Here, we addressed the problem of accurate structural validation with cryo-EM-based methodologies for determining the structures of up to megadalton-scale DNA objects in solution, together with molecular-dynamics-based methods for building pseudoatomic models in a semiautomated fashion. The library of objects includes four brick-like multilayer DNA origami objects with increasing internal floppiness, a barrel-like 126-helix bundle, two variants of a multidomain object called Twisttower, a design variant v2 of a previously reported object called the Pointer, a small 16-helix bundle, four variants of a hinged-beam-like object, two variants of a dumbbell-like object, and five variants of a six-helix tube featuring asymmetric markers at either end as reporters for twist and one ten-helix tube. We constructed pseudoatomic models for six different objects. The fitting was validated using Fourier shell correlation against the cryo-EM half-maps and the models show good cross-correlation with the cryo-EM maps.

The Pointer v2 also exhibited other types of structural fluctuations akin to domain motions. These fluctuations are design-specific and depend on the global shape as well as the topology of the nanostructures. As these motions are driven by the thermal fluctuation of the individual helices, they are also dependent on temperature and salt- and buffer conditions, as well as the overall folding quality of the nanostructure ensemble. The heterogeneity may be coarsely classified as relative domain motions similar to those seen in proteins and as helical lattice breathing, which does not exist in proteins.

> ACAAACGGCGGATTGACCGTAATGGTAACCGTAGAGGCGACCACCACC;> TTTTTCGGATTCTCGACCGTATCGGCTTTTT;> TTGACCCCCAGAGCCACGCCACCCTCAGAACCTTTGCTTTTT;> ACTCATCTAAAGTACAGACTCCTCAAGAGAAG;> ACTAAAACATCCGCGATACGTTGGACGGAGATTTGTATCACGCGAAAC;> AAGAATACTAAAGACTGAACTGACGACCTTCAAAATGCAA;> ACGAAGGCACGGGTAAAAATGTGAGGATATTCAGGTCTTT;> TTTTTCTCAGATGCCACTAGGTTGAGGCCATCTTTTCATAAT;> TTTTTATACCAAGTCGTTTTTTTTTTCCTGATAAATT;> TGTAGATGGGCGCATCGGATAGGTCCTGCTCCATGTTACT;> AATGCTACTACTATTAGTAGAATTGATGCCACCTTTTCAGCTCGCGCCCCAAATGAAAATATAGCTAAACAGGTTATTGACCATTTGCGAAATGTATCTAATGGTCAAACTAAATCTACTCGTTCGCAGAATTGGGAATCAACTGTTACATGGAATGAAACTTCCAGACACCGTACTTTAGTTGCATATTTAAAACATGTTGAGCTACAGCACCAGATTCAGCAATTAAGCTCTAAGCCATCCGCAAAAATGACCTCTTATCAAAAGGAGCAATTAAAGGTACTCTCTAATCCTGACCTGTTGGAGTTTGCTTCCGGTCTGGTTCGCTTTGAAGCTCGAATTAAAACGCGATATTTGAAGTCTTTCGGGCTTCCTCTTAATCTTTTTGATGCAATCCGCTTTGCTTCTGACTATAATAGTCAGGGTAAAGACCTGATTTTTGATTTATGGTCATTCTCGTTTTCTGAACTGTTTAAAGCATTTGAGGGGGATTCAATGAATATTTATGACGATTCCGCAGTATTGGACGCTATCCAGTCTAAACATTTTACTATTACCCCCTCTGGCAAAACTTCTTTTGCAAAAGCCTCTCGCTATTTTGGTTTTTATCGTCGTCTGGTAAACGAGGGTTATGATAGTGTTGCTCTTACTATGCCTCGTAATTCCTTTTGGCGTTATGTATCTGCATTAGTTGAATGTGGTATTCCTAAATCTCAACTGATGAATCTTTCTACCTGTAATAATGTTGTTCCGTTAGTTCGTTTTATTAACGTAGATTTTTCTTCCCAACGTCCTGACTGGTATAATGAGCCAGTTCTTAAAATCGCATAAGGTAATTCACAATGATTAAAGTTGAAATTAAACCATCTCAAGCCCAATTTACTACTCGTTCTGGTGTTCTCGTCAGGGCAAGCCTTATTCACTGAATGAGCAGCTTTGTTACGTTGATTTGGGTAATGAATATCCGGTTCTTGTCAAGATTACTCTTGATGAAGGTCAGCCAGCCTATGCGCCTGGTCTGTACACCGTTCATCTGTCCTCTTTCAAAGTTGGTCAGTTCGGTTCCCTTATGATTGACCGTCTGCGCCTCGTTCCGGCTAAGTAACATGGAGCAGGTCGCGGATTTCGACACAATTTATCAGGCGATGATACAAATCTCCGTTGTACTTTGTTTCGCGCTTGGTATAATCGCTGGGGGTCAAAGATGAGTGTTTTAGTGTATTCTTTCGCCTCTTTCGTTTTAGGTTGGTGCCTTCGTAGTGGCATTACGTATTTTACCCGTTTAATGGAAACTTCCTCATGAAAAAGTCTTTAGTCCTCAAAGCCTCTGTAGCCGTTGCTACCCTCGTTCCGATGCTGTCTTTCGCTGCTGAGGGTGACGATCCCGCAAAAGCGGCCTTTAACTCCCTGCAAGCCTCAGCGACCGAATATATCGGTTATGCGTGGGCGATGGTTGTTGTCATTGTCGGCGCAACTATCGGTATCAAGCTGTTTAAGAAATTCACCTCGAAAGCAAGCTGATAAACCGATACAATTAAAGGCTCCTTTTGGAGCCTTTTTTTTTGGAGATTTTCAACGTGAAAAAATTATTATTCGCAATTCCTTTAGTTGTTCCTTTCTATTCTCACTCCGCTGAAACTGTTGAAAGTTGTTTAGCAAAACCCCATACAGAAAATTCATTTACTAACGTCTGGAAAGACGACAAAACTTTAGATCGTTACGCTAACTATGAGGGTTGTCTGTGGAATGCTACAGGCGTTGTAGTTTGTACTGGTGACGAAACTCAGTGTTACGGTACATGGGTTCCTATTGGGCTTGCTATCCCTGAAAATGAGGGTGGTGGCTCTGAGGGTGGCGGTTCTGAGGGTGGCGGTTCTGAGGGTGGCGGTACTAAACCTCCTGAGTACGGTGATACACCTATTCCGGGCTATACTTATATCAACCCTCTCGACGGCACTTATCCGCCTGGTACTGAGCAAAACCCCGCTAATCCTAATCCTTCTCTTGAGGAGTCTCAGCCTCTTAATACTTTCATGTTTCAGAATAATAGGTTCCGAAATAGGCAGGGGGCATTAACTGTTTATACGGGCACTGTTACTCAAGGCACTGACCCCGTTAAAACTTATTACCAGTACACTCCTGTATCATCAAAAGCCATGTATGACGCTTACTGGAACGGTAAATTCAGAGACTGCGCTTTCCATTCTGGCTTTAATGAAGATCCATTCGTTTGTGAATATCAAGGCCAATCGTCTGACCTGCCTCAACCTCCTGTCAATGCTGGCGGCGGCTCTGGTGGTGGTTCTGGTGGCGGCTCTGAGGGTGGTGGCTCTGAGGGTGGCGGTTCTGAGGGTGGCGGCTCTGAGGGAGGCGGTTCCGGTGGTGGCTCTGGTTCCGGTGATTTTGATTATGAAAAGATGGCAAACGCTAATAAGGGGGCTATGACCGAAAATGCCGATGAAAACGCGCTACAGTCTGACGCTAAAGGCAAACTTGATTCTGTCGCTACTGATTACGGTGCTGCTATCGATGGTTTCATTGGTGACGTTTCCGGCCTTGCTAATGGTAATGGTGCTACTGGTGATTTTGCTGGCTCTAATTCCCAAATGGCTCAAGTCGGTGACGGTGATAATTCACCTTTAATGAATAATTTCCGTCAATATTTACCTTCCCTCCCTCAATCGGTTGAATGTCGCCCTTTTGTCTTTAGCGCTGGTAAACCATATGAATTTTCTATTGATTGTGACAAAATAAACTTATTCCGTGGTGTCTTTGCGTTTCTTTTATATGTTGCCACCTTTATGTATGTATTTTCTACGTTTGCTAACATACTGCGTAATAAGGAGTCTTAATCATGCCAGTTCTTTTGGGTATTCCGTTATTATTGCGTTTCCTCGGTTTCCTTCTGGTAACTTTGTTCGGCTATCTGCTTACTTTTCTTAAAAAGGGCTTCGGTAAGATAGCTATTGCTATTTCATTGTTTCTTGCTCTTATTATTGGGCTTAACTCAATTCTTGTGGGTTATCTCTCTGATATTAGCGCTCAATTACCCTCTGACTTTGTTCAGGGTGTTCAGTTAATTCTCCCGTCTAATGCGCTTCCCTGTTTTTATGTTATTCTCTCTGTAAAGGCTGCTATTTTCATTTTTGACGTTAAACAAAAAATCGTTTCTTATTTGGATTGGGATAAATAATATGGCTGTTTATTTTGTAACTGGCAAATTAGGCTCTGGAAAGACGCTCGTTAGCGTTGGTAAGATTCAGGATAAAATTGTAGCTGGGTGCAAAATAGCAACTAATCTTGATTTAAGGCTTCAAAACCTCCCGCAAGTCGGGAGGTTCGCTAAAACGCCTCGCGTTCTTAGAATACCGGATAAGCCTTCTATATCTGATTTGCTTGCTATTGGGCGCGGTAATGATTCCTACGATGAAAATAAAAACGGCTTGCTTGTTCTCGATGAGTGCGGTACTTGGTTTAATACCCGTTCTTGGAATGATAAGGAAAGACAGCCGATTATTGATTGGTTTCTACATGCTCGTAAATTAGGATGGGATATTATTTTTCTTGTTCAGGACTTATCTATTGTTGATAAACAGGCGCGTTCTGCATTAGCTGAACATGTTGTTTATTGTCGTCGTCTGGACAGAATTACTTTACCTTTTGTCGGTACTTTATATTCTCTTATTACTGGCTCGAAAATGCCTCTGCCTAAATTACATGTTGGCGTTGTTAAATATGGCGATTCTCAATTAAGCCCTACTGTTGAGCGTTGGCTTTATACTGGTAAGAATTTGTATAACGCATATGATACTAAACAGGCTTTTTCTAGTAATTATGATTCCGGTGTTTATTCTTATTTAACGCCTTATTTATCACACGGTCGGTATTTCAAACCATTAAATTTAGGTCAGAAGATGAAATTAACTAAAATATATTTGAAAAAGTTTTCTCGCGTTCTTTGTCTTGCGATTGGATTTGCATCAGCATTTACATATAGTTATATAACCCAACCTAAGCCGGAGGTTAAAAAGGTAGTCTCTCAGACCTATGATTTTGATAAATTCACTATTGACTCTTCTCAGCGTCTTAATCTAAGCTATCGCTATGTTTTCAAGGATTCTAAGGGAAAATTAATTAATAGCGACGATTTACAGAAGCAAGGTTATTCACTCACATATATTGATTTATGTACTGTTTCCATTAAAAAAGGTAATTCAAATGAAATTGTTAAATGTAATTAATTTTGTTTTCTTGATGTTTGTTTCATCATCTTCTTTTGCTCAGGTAATTGAAATGAATAATTCGCCTCTGCGCGATTTTGTAACTTGGTATTCAAAGCAATCAGGCGAATCCGTTATTGTTTCTCCCGATGTAAAAGGTACTGTTACTGTATATTCATCTGACGTTAAACCTGAAAATCTACGCAATTTCTTTATTTCTGTTTTACGTGCTAATAATTTTGATATGGTTGGTTCAATTCCTTCCATAATTCAGAAGTATAATCCAAACAATCAGGATTATATTGATGAATTGCCATCATCTGATAATCAGGAATATGATGATAATTCCGCTCCTTCTGGTGGTTTCTTTGTTCCGCAAAATGATAATGTTACTCAAACTTTTAAAATTAATAACGTTCGGGCAAAGGATTTAATACGAGTTGTCGAATTGTTTGTAAAGTCTAATACTTCTAAATCCTCAAATGTATTATCTATTGACGGCTCTAATCTATTAGTTGTTAGTGCACCTAAAGATATTTTAGATAACCTTCCTCAATTCCTTTCTACTGTTGATTTGCCAACTGACCAGATATTGATTGAGGGTTTGATATTTGAGGTTCAGCAAGGTGATGCTTTAGATTTTTCATTTGCTGCTGGCTCTCAGCGTGGCACTGTTGCAGGCGGTGTTAATACTGACCGCCTCACCTCTGTTTTATCTTCTGCTGGTGGTTCGTTCGGTATTTTTAATGGCGATGTTTTAGGGCTATCAGTTCGCGCATTAAAGACTAATAGCCATTCAAAAATATTGTCTGTGCCACGTATTCTTACGCTTTCAGGTCAGAAGGGTTCTATCTCTGTTGGCCAGAATGTCCCTTTTATTACTGGTCGTGTGACTGGTGAATCTGCCAATGTAAATAATCCATTTCAGACGATTGAGCGTCAAAATGTAGGTATTTCCATGAGCGTTTTTCCTGTTGCAATGGCTGGCGGTAATATTGTTCTGGATATTACCAGCAAGGCCGATAGTTTGAGTTCTTCTACTCAGGCAAGTGATGTTATTACTAATCAAAGAAGTATTGCTACAACGGTTAATTTGCGTGATGGACAGACTCTTTTACTCGGTGGCCTCACTGATTATAAAAACACTTCTCAAGATTCTGGCGTACCGTTCCTGTCTAAAATCCCTTTAATCGGCCTCCTGTTTAGCTCCCGCTCTGATTCCAACGAGGAAAGCACGTTATACGTGCTCGTCAAAGCAACCATAGTACGCGCCCTGTAGCGGCGCATTAAGCGCGGCGGGTGTGGTGGTTACGCGCAGCGTGACCGCTACACTTGCCAGCGCCCTAGCGCCCGCTCCTTTCGCTTTCTTCCCTTCCTTTCTCGCCACGTTCGCCGGCTTTCCCCGTCAAGCTCTAAATCGGGGGCTCCCTTTAGGGTTCCGATTTAGTGCTTTACGGCACCTCGACCCCAAAAAACTTGATTTGGGTGATGGTTCACGTAGTGGGCCATCGCCCTGATAGACGGTTTTTCGCCCTTTGACGTTGGAGTCCACGTTCTTTAATAGTGGACTCTTGTTCCAAACTGGAACAACACTCAACCCTATCTCGGGCTATTCTTTTGATTTATAAGGGATTTTGCCGATTTCGGAACCACCATCAAACAGGATTTTCGCCTGCTGGGGCAAACCAGCGTGGACCGCTTGCTGCAACTCTCTCAGGGCCAGGCGGTGAAGGGCAATCAGCTGTTGCCCGTCTCGCTGGTGAAAAGAAAAACCACCCTGGCGCCCAATACGCAAACCGCCTCTCCCCGCGCGTTGGCCGATTCATTAATGCAGCTGGCACGACAGGTTTCCCGACTGGAAAGCGGGCAGTGAGCGCAACGCAATTAATGTGAGTTAGCTCACTCATTAGGCACCCCAGGCTTTACACTTTATGCTTCCGGCTCGTATGTTGTGTGGAATTGTGAGCGGATAACAATTTCACACAGGAAACAGCTATGACCATGATTACGAATTCGAGCTCGGTACCCGGGGATCCTCTAGAGTCGACCTGCAGGCATGCAAGCTTGGCACTGGCCGTCGTTTTACAACGTCGTGACTGGGAAAACCCTGGCGTTACCCAACTTAATCGCCTTGCAGCACATCCCCCTTTCGCCAGCTGGCGTAATAGCGAAGAGGCCCGCACCGATCGCCCTTCCCAACAGTTGCGCAGCCTGAATGGCGAATGGCGCTTTGCCTGGTTTCCGGCACCAGAAGCGGTGCCGGAAAGCTGGCTGGAGTGCGATCTTCCTGAGGCCGATACGGTCGTCGTCCCCTCAAACTGGCAGATGCACGGTTACGATGCGCCCATCTACACCAACGTAACCTATCCCATTACGGTCAATCCGCCGTTTGTTCCCACGGAGAATCCGACGGGTTGTTACTCGCTCACATTTAATGTTGATGAAAGCTGGCTACAGGAAGGCCAGACGCGAATTATTTTTGATGGCGTTCCTATTGGTTAAAAAATGAGCTGATTTAACAAAAATTTAACGCGAATTTTAACAAAATATTAACGTTTACAATTTAAATATTTGCTTATACAATCTTCCTGTTTTTGGGGCTTTTCTGATTATCAACCGGGGTACATATGATTGACATGCTAGTTTTACGATTACCGTTCATCGATTCTCTTGTTTGCTCCAGACTCTCAGGCAATGACCTGATAGCCTTTGTAGATCTCTCAAAAATAGCTACCCTCTCCGGCATTAATTTATCAGCTAGAACGGTTGAATATCATATTGATGGTGATTTGACTGTCTCCGGCCTTTCTCACCCTTTTGAATCTTTACCTACACATTACTCAGGCATTGCATTTAAAATATATGAGGGTTCTAAAAATTTTTATCCTTGCGTTGAAATAAAGGCTTCTCCCGCAAAAGTATTACAGGGTCATAATGTTTTTGGTACAACCGATTTAGCTTTATGCTCTGAGGCTTTATTGCTTAATTTTGCTAATTCTTTGCCTTGCCTGTATGATTTATTGGATGTT;> TTTTTAAGGTGGCATCAATTCTACAAAGCGGAGACTTCAA;> TTTTTATAAATCACGAGCTTCAAGGATTTTT;> ATATTTTCATTTGGGGAATAACCTCTCCAACATTTTGATA;> TTTTTCGCAAATGGTCCGCGAGCTGCCCGAAATTGCATCATATTATAG;> TTTTTAAATTAAGGATGGCTTATTTCTTTTT;> ATTCTGCGCTGTAGCTTGTCTGGATCAATCATAAATATTT;> TTTTTTAAATCGGTTTGCGGGAGAAGTTTTT;> ATGACCCTGTAATACTTTGTACCACCTCAGAGCATAAAGCTTTTT;> AAGTACGGCAACATGTGTCATTGCTGCCGGAGAGAACTGG;> TTTTTTGCAACTAACATTTTTTTTTTGTTGATTCCCATAGATACA;> TTTTTCCTTTAGAGCTTAAATCGATGGAGGCTTTTT;> ATTGCTGATTTTTGCGCAATAAAGAGGCAAAGAATTAGCATTTTT;> ATCTGGTGAACGAGTAAAAACATTAGTTTCATTCCATGTA;> ATTGCTCCGGTCAGGATAAATTAAAGACAGTCAGCTGCTC;> TTTTTAACGCAAAGCGAAAATACTGCGGAATTTTTT;> CCAGACCGTTTTAATTTACAGGCAGTAGCATTAACATCCATTTTT;> TTAGAGAGTTTTTTTTTTTACCTTTATTTTTTTT;> TTTTTTAAAAATTTTTAGTAATGTGTTAAATTTTTT;> AAAAGATTTTTTTTTTTTAAGAGGAAGAATTTTT;> TTTTTATCATTTTTCATTTTTTTTTTTCAACATT;> TTTTTATTCATTGAATCCAAAGAGGAGTGTCGAA;> GAAAACGACAATCATATAGCCGGAAAAACGAA;> TTTTTCGTCAAGGTAAAGACGAGAACGGCGCATAGCAGCGAA;> ATTCAAAATGCCTGAGAACCCTCATATATTTTTAATAGTA;> GGGTGAGAATATCGCGGAAGCAAAGTTTAGCTGATTTAGTTTGACCAT;> AAGGCCGGAAATGTTTTTAATCATCTCATTATGGGCCTCT;> ATCAATATGATTTTTTTTTTTATTTCCTGTAGTTTTT;> TTTTTTTTTGCAAAAGAAGGAAGAAAGCTTGAGAGCTGCGCAAGCTTGAT;> TAATAGTACTGAGAGTAGAAAGATAAAAGGAATGCTAAAC;> TATTTTTGAGATTTTTTTTTTGATCACCGCCATTTTT;> CAAAAACAGGAAGATTGTATAAGCATGTACCCATAACGCCTCATCAGT;> TTTTTAGCGAAACGGTAAGAGCAACATAACGGAAAAAAAAAG;> AATCAGAAAAGTTTTTTTTTTCCCTAACCAATTTTTT;> GCAGATACCGGTTGATGCTATCAGTTTAAATATTTTT;> TTTTTAGGAAATTGAGAATAGGGGTTTTTTT;> TTTTTCTCGTTTACCAGACGACGACGTAACGAAAATGAAT;> TAAAATTCAAATTGTAAACGTTAATAAAAACCAAAATTTTTT;> GCGTTAAATTTTTGTTCCAGTGCCAACTTTCACCCAATAG;> TTATTTTTTTTTTATAAAACGAACCTATCATAACGTTAGT;> AATCTACGATCGGTTTGCTCCAAATTGATATA;> TTTTTTCAAAAATGGGGGATGAAAGGAACCAGAACCG;> ACCAGAACTCTTAAACATCAGCTTCAGGGTGGAGAGGCGG;> AATAAGGCTTTCAACTAGACTGGAAGAGGGGGAGAGGTCA;> TTTTTCCAGCACCGATATATTCTCCATTTTT;> TGTGAATTGGAAACCAAACAACCAGTTGAGTG;> CAGATGAAAACGGCTAAGACAGCAGGGCGAAA;> CAACTTTGCCCTCAAATGCTTTAAACAGTTCATCAGAAGC;> AGGGAACCTTTTCATGGCTTTTGCACTACGTGTTGTTCCA;> CAGACGGTGAATGACCATAAATCAAAATTTTT;> TCAAGAGTATTCAGTGACAATGACGGCAAAGCGCAACAGC;> AATCTTGATAAAGGCCAGGAAGTTCCGGAACCAGAGCCGC;> CGCTTTTTTTTTTGTTTTCATCGGCATTTTCGGTCATAGC;> TTTTTGATTGGCCTTGATATTCACTGTACTGGTAATATTTTT;> TTTTTGGGGTGCCACCCTCAGCGATTTTTTT;> GTATAAACAGTTAATGCCCCCTGCAGAGCCGCGTCTCTGA;> CAGTGCCCACATGGCTTTTGATGATACAGGAGAAACGAATTTGACAGG;> TTTTTAGTTTTAACGGGGTCAGTGCCTTGAGTAACGCCAGCAGGATCTTC;> TTTTTAACATGAAGATTAGGATTAGCTTTTT;> AGTATTAAGAACCTATTATTCTGATTTTT;> GAGGCTGAATTTACCGTTCCAGTAAAAGCGCACACCAGAA;> AAGGGAAGGTCTGTCCGTTTGGAACGAGACGGGCCATTCG;> GCATCTGCATTAAAGCCAGAATGGAGCGTCAT;> CAGTTTGAGGGGACGACCGTGGGAGCGAGTAACAACCCGTTTTTT;> TTTTTAGGGTAGCCGGTTTTTTTTTTTGTACAGACCA;> CAGAGGCTCTCAGAGCCCACCCTCCTATTTCG;> AATACGTAGAAGATTTTTTTTTTTCGCACGGTCGCT;> TTTTTGCCAGCTTTCCGGTGAGAGAGGCCCGCTTATTACGCA;> TTTTTGGTGAATTGAGTTTTTTTTTTTAGTAAATTGG;> ATCTCCAACAACATTAGGACGTTGGTTTTGCCTAGCGTCC;> TTTTTTCAACCGTACTGAACCCATTACCGAAC;> AATAATAATCGCTATTGTCGTGCCTGATTGCCATCCAGAA;> AACTAAAGAGCGGAGTCAACTAATTCATTTTT;> TTTTTTAGTTGGGTAACGCCATGCTGCAACGCTCACT;> ACTGTTGGGCGCGGGGTTTTTCTTCAGGAAAA;> GAAGGGCGCCATTCAGTGGTTTAATTGCCCTG;> ATCGGTGCACCAGTCATTACAGGTCTGGAGCACTAGCATG;> ACGCCAGCCTGGTGCCACCTTATGCGTAACAAAAATCACCACCCTGAC;> TGGCGAAAAATTCGCGAGGAATACCTACAAAG;> TCTAAAGTAACGCCTGTAGCATTCAATATCAAGCCCTAAA;> ATGCCCTCATAGTTAGTATTTTGTCATAGTAATCGTAAAAAACAAGAG;> AAGCTTGCGTCGACTCTAGAGGATAAAAATCTGAACCACC;> TTTTTTTCCCAGTCACGACGAATTCGTAATCATGAACAGTGC;> ACAGTTTCGAATTGCGTGAGATTTCGATTTTAAGGGTAGCCTAGCTGA;> AACTTTTTTTTTACTTTGTCGTTTTTTTTTTTCTTTCCAGACCTTTTT;> CCAGTACAAACTGATAACCTTTTTTTTTTCTCAATCAATA;> TTTCGTCAAGTATAGCCCCTTCTGACATTCTGATTTACAT;> ACCCTCATGAGGTGAGCACGCTGACTAAAATATCTTTAGG;> CACCCTCAGAGCCACCCCACCCTCAAGTAAGCGTATGTTA;> CACAACATAAACGATTATTATTTAGCCAGTTACAAAATAA;> ACCGAGCTCGTTGTAAAACGACGGAAATCAGC;> CGCTTTTTTTTTTTCACAATTCCAAGCCTGGGAATAGCTA;> AGCTGCATACCCAAAAGAGGAAACAATTGAGCACACCCTG;> TTTTTGCCGTCGAGAGGGAGGAGCCTTTTTTTTTTTTTAATTGT;> GGTGTATCCGTTGAAATGGGGTTTTTACGAGG;> CAGGAGGTAGGAAACCGAACTGGCTACCAGCGAGGGAGGG;> GTGTTTTTTTTTTCCTAATGAGTGGCAGGCGATTGGGAAT;> GGACTCCAACCAGTTTTTTTTTTGCGGATTGGGCGCGCTTTCGATTTTT;> AAGAACGTTCAGTGAGACGCTCATGGAAA;> CACTATTAAACCGTCTAGGAGCGGGCGCTAGGGCGCTTTTTT;> TTCACCAGCAAGAGTCACCGATAGCACCCTCAGGCTGGCT;> CTTCACCGGAGATAGGTCGCCCACCAGGGAGTCAAGAACC;> TTGCAGCAGAAGAACTGTAATAACGTGCTTTC;> ACGCTGGTTTGCCCCAAGCTAACTCATACATATCTTACCG;> AAATTTTTTTTTTTCCTGTTTGATGACTGTAGGAATCAAGTTTGCCTT;> AGAGCCACCACCGGAAGATGGCCCGGGATCGTTTGCGCCG;> TTTTTTCAGTACGTCAAATCGGAACGTTTTT;> AACCATCAAACGTGGCGAGAAAGGCCCGCCGCGGCCGATTTACATCGG;> CCCAAATCCAAAATCATCCATTAAACCAACCTACGAGGCG;> AAGTTTTTGAGGCTTGGCATAACCCAAATCAATCTGGCCTCAACCGTT;> TGGGGTCGATCAAAAGTTTGATTACAAACTATGAAATTAT;> AGGTGCCGCCCGATTTAGAGCTTGGTACTATGCTCGTTGG;> TAAAGCACCCCCTTATTAGCGTTTGCAGGTCAGACTTTTT;> TAAATCGGTAGCGTCAGGTGGTTCCACCATTATAGAGCCA;> GAAGGCTTGAGAAACAAGTTGAGTATATGTACTCATATGCGTTATACA;> CAGATATAAAGGTAAACGGGAGCTGTTGTAGCAGCCGGCG;> GGAATCATGGTGAATTCGTATAACATCACTTGAGGGAGCC;> TTTTTGCCGTTTTTATTTAGCATGTATTTTT;> AGAACGGGCCAATAGCATCAAAATCATAGGTCTTGGGTTA;> TTGCTTCTAGCTTAGATTCTAAGACGGGAGGTAAAAGGGC;> TTTTTGAAACCAATTTTTTTTTTTTTACGTAACCTCCGGCTTAGG;> TTTTTCCTTAGATTTTTTTTTTTTTTCAGGTTTA;> ATAGCGATGTAAATCGCAGTAACATTTAACAAGCGCGTAACCACCACA;> AGTCAATAGAATACCAATAACGGAAAACAAACCGCCGCTACAGGGCGC;> ACGGGGAAAATACTTCAATAGCCCCCTGGCCCCACCGCTT;> TTTTTGGCAAGTGTAGCGACGCCAGAACGTCAGA;> GTTGCTTTTTACCTGAGCAAAAGAGAATTATTTCATTCCA;> GACGAGCAGCAGCACCAACCCTAAACCAGTAGCGAAATCG;> GTAATCAGAATGAAACCGAGAACAAGCAATTTTT;> ATCTTGAGAAGTTTTTTTTTTTGTTTTTATAA;> AAAGGGATGACATTCACCGCCAGCAACGGAATTAATGAAT;> GCCACCGAGGAACGGTGTCACGCTTTTCATTTGAATTTTT;> GTAAAAGAAAAGCGAAATCAGGGCCCGCCTCCTTGAGGAC;> ATCACGCACAATATTAACCGATTGCTAAAGACTTTGAAGC;> AATTAACCAAACAGGAGCTTAATGATCAAGAAAACAAAAT;> CCATTAGCAAGGCTTTTTTTTTTCGGAAACGTCACCTAGCGACA;> TACCTACATTTTGTGGCAGATTCACCAGTCACTTTTT;> ACGCTCAACGTTTTAGTGAATATATCGCTATTCCTTTTTT;> TATTGACGCGGCCTTGGACTCCTTTCCAGTCGGCCACCCT;> ATCACCGTGCAAAATCAGAAAATACACATTAAGAAGCATAAAGTGTAA;> CACCGACTAAAGACACACCAACGCTAACGTTTTT;> GAAAATTCTAACCCACGAACAAAGATAAAACATTTCAGGG;> AATCAATATTGCACCCGATTATACTTCTGAATACCACCAG;> TTTGTCACTCATTAAATACCGCGCTATTAAACTTTCCTTACATTTCAA;> AAGTTTATGCAAACGTCCTGAGTAAGCGGTCCGCAAAATCCCTTATAA;> TTTTTACGACCAGTAATTTGCGTATAAGTTTTTT;> TAAAAGGGACCTGAAAGCGTATTTTT;> AAGGTGGCAACATTTTTTTTTTTATAAAAGAAACGCTGAGCCAT;> AGATAGCCAAGAATTGAGGGAAGCAAGGAGCG;> TTTTTAGAATACGTGGCAAATGCGCG;> CAGAGGGTGCAATAATATTAAAAAGTACCGTAACCTGCAG;> GAAACAATAGCAGCCTTCAGATGACTTTCTTTTT;> TAGTCTTTCAGACAATCGTAAAACAGAAATTTTT;> ATGGCTATACATCGCCAGATAGAACCGGAATACGGCCAAC;> TTAACTGAGCTAATATGAATTGAACTTAAATCAAGATTAG;> CGGGAGAAAGCAGAAGTTACCAGATTAGTACCGGAAACCT;> GCATTAGAAAGGTTATGAGCCAGCAGCAAATGCCCCGGGTATAGCAAG;> GCGGTCAGATAAAAACAGTTAAGCATTGTTTGAGCTACAATTTTATCC;> TATTAACATTTAAGAAAGAACCGCTTGCGTTGGGCGATTATTTTTT;> CAAATAAGACGAGCCGTGTTTCCTGTGTGAAATTGTTATCACAGCCAT;> TTTTGTTTAACGTTTTTTTTTTTCAAAAATGAAAATGAAATAGC;> ACCTTGCTGAACCTCACACAGACAACACTGAGTTTCTGTA;> AAAGCATCATCAACAGTAGAAAGGGACTTTACTTTGCGGAACAAAGAA;> CAACTAATTCCCAATCCCGCCTGCGTCATAGC;> ATCCTTTGCCCGATTTTTTTTTTACGTTATTAATTTTAAAAGTT;> ACATTTGAGGATTTAGAAGTATTAAATTGAGG;> TAGATAATGAATTATCATCATATTTAATCCTGCCAATAAT;> TTTTTCAGAGCCTAATTTAGATTAGAGCCGTCAATGCACTAAAGAATAAC;> ATTATCATAAACAATTCGACAACTCGTATTAATCTGGTCA;> TATTAGCAATTTTTGAAATGGATTGCCAACAGCATTGCAA;> CCAACCATATCAAAATTGAGTAACAACAAAGTGTTGGCAA;> TATGGAAGCAGAGAGAATATGGTTATGATTAACTGGTAAT;> TTTTTAGCGTTGGCAATTCATCAATACCTGATTATTACAGAG;> TTTTTTAAAGCGAACCTCCCGACTTGACGCGAGGTCGTCTGATTTAGACA;> AAATTGCGTAGAATCCTTGAAAACAACTTTTTCAAATTTTTT;> ATCCGGTATTAAGACGCTGAGAAGCAAATCCAGCCTGTTT;> TGAGAGACCGGCTGTCCAAGTACCGCACTCATCATCGATA;> TACCTTTTTCATCGTATGAATCTTCACGGAATAAGAGCAAAAGCCCTT;> TTTTTATATTTTAGTTAAGTAGGGCTTTTTT;> TAGATAAGATTGCTTTGTGAATTTAAGCAAATTTGCTATT;> TCCTGAACTATAACTATCGAGCCAGTAATAAGAGAATATAAAGTATTTTT;> AAGAAAAAAAGTAATTAACACCGGTTTTTTTTTTAATCATAATTACTAGA;> ACATGTTCCCGTGTGATAAATAAGGCGTTAAAAAAAGCCT;> TTTTTCCGACAAAAGGTATAATATCCCATCCTAATCAATAAT;> TTTTTTAATTGAGAATCGCCAGCTCAACATTTCATCT;> AACGCCAACATGTAATTTAGGCAGAATAAACAATCAACAAGTTTAGTA;> CCAGTATAAATGGAAACAGTACATTAATTACAGTACCTTT;> AAGCCAACTGGTTTGAAATTCTTATCTGACCT;> AATACCGAAGCTAATGAAATTTAATATTTAACACAAAGAACGCGAGAA;> TAAGAATACTGTCCAGACGACGACAGGCATTTTATGTAAATGCTGATG;> TTTTTTTAAATTAATTTTCTTTTT;> AAATCAATGAATAACCCAGAACGCATCGCAAG;> AAAATCGCGCAGAGGCAGATGATGTTCGCCTGAATCAGAG>MIEERLEALQSESHRLENALSIIEEERKQLKLKEAELQEEYQNSLRPLQQLQYLTLSACEEEKRQELMYEIGQIGDLIEDWATDKREALKREEGRIEDKQNELFYKRQKLILEVEEQKKDKESTDG[4x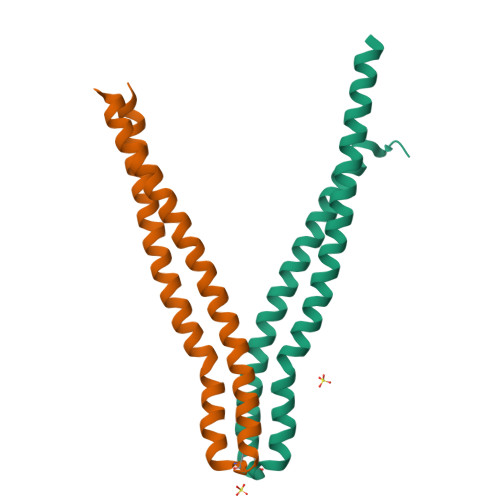]>PISPIETVPVKLKPGMDGPKVKQWPLTEEKIKALVEICTEMEKEGKISKIGPENPYNTPVFAIKKKDSTKWRKLVDFRELNKRTQDFWEVQLGIPHPAGLKKKKSVTVLDVGDAYFSVPLDEDFRKYTAFTIPSINNETPGIRYQYNVLPQGWKGSPAIFQSSMTKILEPFKKQNPDIVIYQYMDDLYVGSDLEIGQHRTKIEELRQHLLRWGLTTPDKKHQKEPPFLWMGYELHPDKWTVQPIVLPEKDSWTVNDIQKLVGKLNWASQIYPGIKVRQLCKLLRGTKALTEVIPLTEEAELELAENREILKEPVHGVYYDPSKDLIAEIQKQGQGQWTYQIYQEPFKNLKTGKYARMRGAHTNDVKQLTEAVQKITTESIVIWGKTPKFKLPIQKETWETWWTEYWQATWIPEWEFVNTPPLVKLWYQLEKEPIVGAETFYVDGAANRETKLGKAGYVTNKGRQKVVPLTNTTNQKTELQAIYLALQDSGLEVNIVTDSQYALGIIQAQPDKSESELVNQIIEQLIKKEKVYLAWVPAHKGIGGNEQVDKLVSA[4x];>IETVPVKLKPGMDGPKVKQWPLTEEKIKALVEICTEMEKEGKISKIGPENPYNTPVFAIKKKDSTKWRKLVDFREL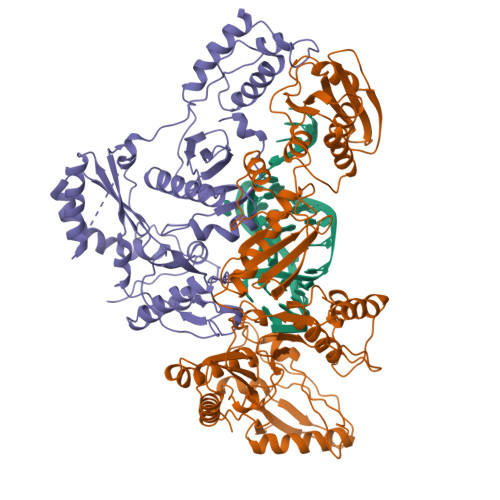NKRTQDFWEVQLGIPHPAGLKKKKSVTVLDVGDAYFSVPLDEDFRKYTAFTIPSINNETPGIRYQYNVLPQGWKGSPAIFQSSMTKILEPFKKQNPDIVIYQYMDDLYVGSDLEIGQHRTKIEELRQHLLRWGLTTPDKKHQKEPPFLWMGYELHPDKWTVQPIVLPEKDSWTVNDIQKLVGKLNWASQIYPGIKVRQLCKLLRGTKALTEVIPLTEEAELELAENREILKEPVHGVYYDPSKDLIAEIQKQGQGQWTYQIYQEPFKNLKTGKYARMRGAHTNDVKQLTEAVQKITTESIVIWGKTPKFKLPIQKETWETWWTEYWQATWIPEWEFVNTPPLVKLWY[4x]> GAMGSHLQAPTWYGEPSPAAHWAFGGKLVQITPDGKGVSITNPKISGLESNTTLSEALKTKDFKPLINQRLVKVIDDVNEEDWNMLEKLSMDGTEEFLKEALAFDNDESDAQDDANNEKEDDGEEFFQQIETNFQPEGDFSLSGNIEQTISKNLVSGNIKSAVKNSLENDLMMEAMVIALDSNNERLKESVKNAYFAKYGSKSSLSRILYSISKREVDDLVENLDVSQWKFISKAIQNLYPNDIAQRNEMMIKLGDRMKENGHRQDSLTLYLAAGSLDKVASIWLSEFPDLEDKLKKDNKTIYEAHSECMTEFIERFTVFSNFINGSSTINNEQLIAKFLEFINLTTSTGNFELATEFLNSLPSDNEEVKTEKARV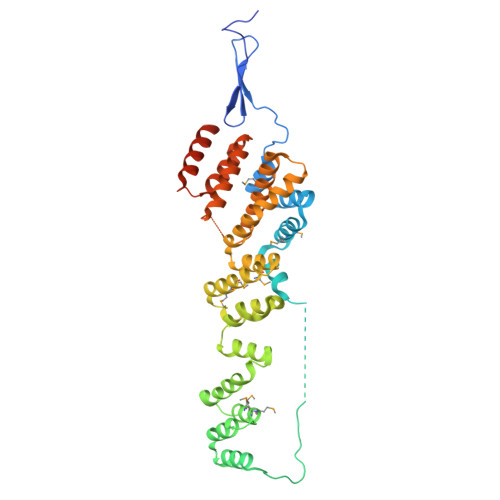LIASGKSLPAQNPATATTSKAKY>MGSDKIHHHHHHMEFEVKKTFGKARLGVMKLHHGAVETPVFMPVGTNASVKLLTPRDLEEAGAEIILSNTFHLMLKPGVEIIKLHRGLHNFMGWKRPILTDSGGFQVFSLPKIRIDDEGVVFRSPIDGSKVFLNPEISMEVQIALGSDICMVFDHCPVPDADYEEVKEATERTYRWALRSKKAFKTENQALFGIVQGGIYPDLRRESALQLTSIGFDGYAIGGLSIGEERSLTLEMTEVTVEFLPEDKPRYFMGGGSPELILELVDRGVDMFDSVFPTRIARHGTALTWNGKLNLKASYNKRSLEPV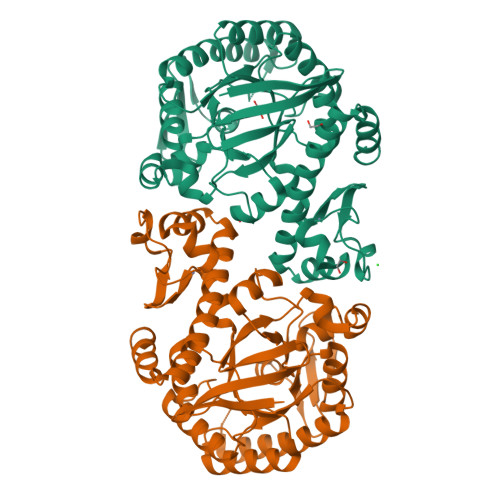DERCGCYTCKNFTRSYIHHLFDRGEVLGQILLTIHNINFMISLMKEVRRSIESGTFKELKSKVVEVYSSGGVNV[4x]>MDIKYKLASYRICSPEETFEKIQEALKKIETVEIKNIQHLDKVNIPVYYLKRRVVVDGKEGIAIHYGKGANDIQAKVSACMEAIERFSASYDKNKVKEKPDNPINVEDLILPQYADKNVKEWVEGIDIINNETIDVPADAVFYPTSGKLFRGNTNGLASGNNLDEAILHATLEIIERDAWSLADLARKIPTKINPEDAKNPLIHELIEKYEKAGVKIILKDLTSEFEIPVVAAISDDLSKNPLMLCVGVGCHLHPEIAILRALTEVAQSRASQLHGFRRDAKLREEFTSKIPYERLKRIHRKWFEFEGEINIADMPNNARYDLKKDLKFIKDKLSEFGFDKLIYVDLNKVGVDAVRVIIPKMEVYTIDRDRLSRRAFERVKKLYY[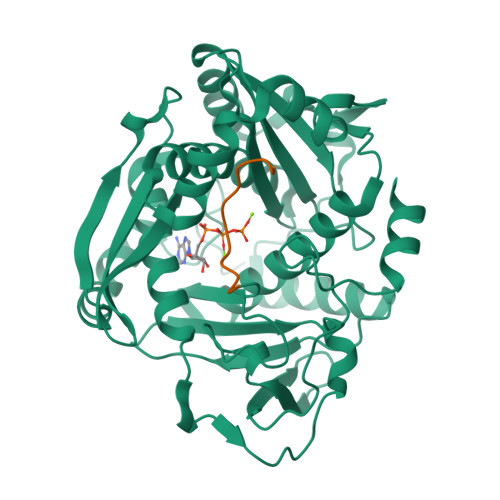4x];>[4x]GRLGFYGYDLQD>[4x]MRKIVVAAIAVSLTTVS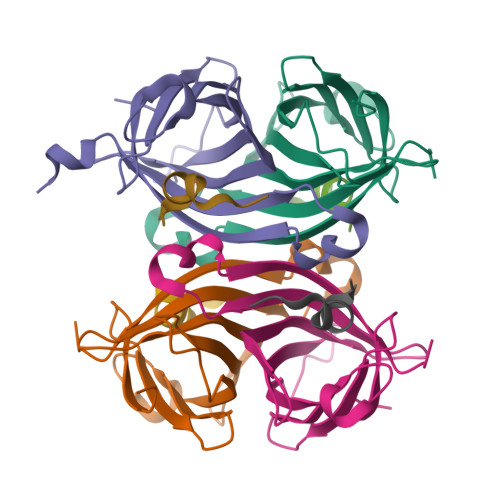ITASASADPSKDSKAQVSAAEAGITGTWYNQLGSTFIVTAGADGALTGTYESAVGNAESRYVLTGRYDSAPATDGSGTALGWTVAWKNNYRNAHSATTWSGQYVGGAEARINTQWLLTSGTTEANAWKSTLVGHDTFTKVKPSAASIDAAKKAGVNNGNPLDAVQQ;>[4x]AFPDYLAEYHGGX>MFFNKKNNQDELKKLAATEAAKSITTEITLGVGTGSTVGFLIEELVNYRDKIKTVVSSSEDSTRKLKALGFDVVDLNYAGEIDLYIDGADECNNHKELIKGGGAALTREKICVAAAKKFICIIDESKKVNTLGNFPLPIEVIPMARSYIARQIVKLGG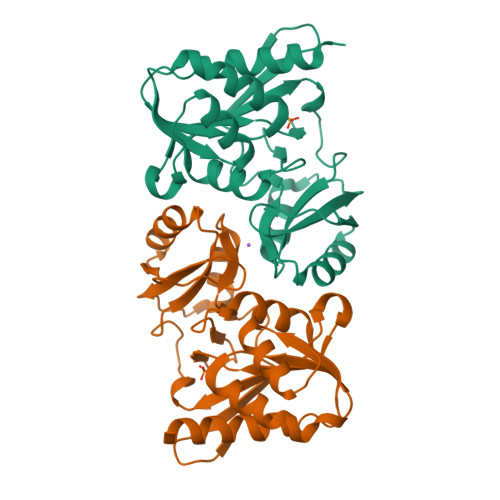QPVYREQTITDNGNVILDVYNLKIDNPLKLETELNQITGVVTNGIFALKPADTVIMATKDSNIVVL[4x]> MTEFWLISAPGEKTCQQTWEKLHAATTKNNNLAVSSKFNIPDLKVGTLDVLVGLSDELAKLDAFVEGVVKKVAQYMADVLEDSKDKVQENLLASGVDLVTYITRFQWDMAKYPIKQSLKNISEIIAKGVTQIDNDLKSRASAYNNLKGNLQNLERKNAGSLLTRSLAEIVKKDDFVLDSEYLVTLLVVVPKLNHNDWIKQYETLAEMVVPRSSNVLSEDQDSYLCNVTLFKKAVDDFRHKARENKFIVRDFQYNEEEMRADKEEMNRLSTDKKKQFGPLVRWLKVNFSEAFIAWIHIKALRVFVESVLRYGLPVNFQAMLLQPNKKSVKKLREVLHELYKHLDSSAAAIIDAPMDIPGLNLSQQEYYPYVYYKIDCNLLEFK;>M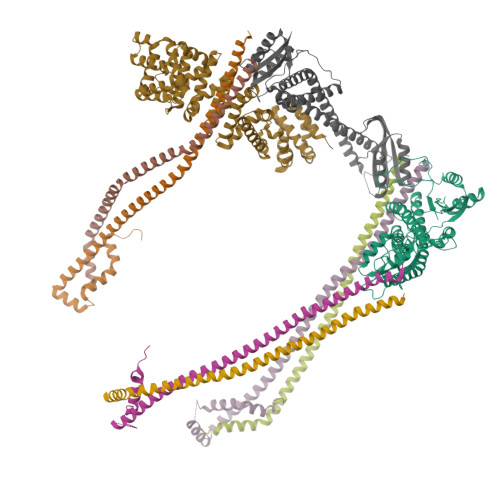ALSDADVQKQIKHMMAFIEQEANEKAEEIDAKAEEEFNIEKGRLVQTQRLKIMEYYEKKEKQIEQQKKIQMSNLMNQARLKVLRARDDLITDLLNEAKQRLSKVVKDTTRYQVLLDGLVLQGLYQLLEPRMIVRCRKQDFPLVKAAVQKAIPMYKIATKKDVDVQIDLEAYLPEDIAGGVEIYNGDRKIKVSNTLESRLDLIAQQMMPEVRGALFGANANRKFLD[3x];>[3x]MASQSQGIQQLLQAEKRAAEKVADARKRKARRLKQAKEEAQMEVEQYRREREQEFQSKQQAAMGSQGNLSAEVEQATRRQVQGMQSSQQRNRERVLTQLLGMVCDVRPQVHPNYRITV;> MTKMDIRGAVDAAVPTNIIAAKAAEVRANKVNWQSYLQGQMISAEDCEFIQRFEMKRCSEEKQEMLQTEGSQCAKTFINLMTHISKEQTVQYILTMVDDMLQENHQRVSIFFDYAKRSKSTAWPYFLPMLNRQDPFTVHMAARIIAKLAAWGKELMEGSDLNYYFNWIKTQLSSQKLRGSGVAVETGTISASDSSQYVQCVAGCLQLMLRVNEYRFAWVEADGVNCIMGVLSNKCGFQLQYQMIFSIWLLAFSPQMCEHLRRYNIIPVLSDILQESVKEKVTRIILAAFRNFLEKSTERETRQEYALAMIQCKVLKQLENLEQQKYDDEDISEDIKFLLEKLGESVQDLSSFDEYSSELKSGRLEWSPVHKSEKFWRENAVRLNEKNYELLKILTKLLEVSDDPQVLAVAAHDVGEYVRHYPRGKRVIEQLGGKQLVMNHMHHEDQQVRYNALLAVQKLMVHNWEYLGKQLQSEQPQTAAARS;> MGELFRSEEMTLAQLFLQSEAAYCCVSELEELGKVQFRDLNPDVNVFQRKFVNEVRRCEEMDRKLRFVEKEIRKANIPIMDTGENPEVPFPRDMIDLEANFEKIENELKEINTNQEALKRNFLELTELKFILRKTQQFFDEMADPDLLEESSSLLEPNEMGRGAPLRLGFVAGVINRERIPTFERMLWRVCRGNVFLRQAEIENPLEDPVTGDYVHKSVFIIFFQGDQLKNRVKKICEGFRASLYPCPETPQERKEMASGVNTRIDDLQMVLNQTEDHRQRVLQAAAKNIRVWFIKVRKMKAIYHTLNLCNIDVTQKCLIAEVWCPVTDLDSIQFALRRGTEHSGSTVPSILNRMQTNQTPPTYNKTNKFTHGFQNIVDAYGIGTYREINPAPYTVITFPFLFAVMFGDFGHGILMTLFAVWMVLRESRILSQKNENEMFSMVFSGRYIILLMGLFSIYTGLIYNDCFSKSLNIFGSSWSVRPMFTIGNWTEETLLGSSVLQLNPAIPGVFGGPYPFGIDPIWNIATNKLTFLNSFKMKMSVILGIIHMLFGVSLSLFNHIYFKKPLNIYFGFIPEIIFMSSLFGYLVILIFYKWTAYDAHSSRNAPSLLIHFINMFLFSYPESGNAMLYSGQKGIQCFLIVVAMLCVPWMLLFKPLILRHQYLRKKHLGTLNFGGIRVGNGPTEEDAEIIQHDQLSTHSEDAEEPTEDEVFDFGDTMVHQAIHTIEYCLGCISNTASYLRLWALSLAHAQLSEVLWTMVIHIGLHVRSLAGGLGLFFIFAAFATLTVAILLIMEGLSAFLHALRLHWVEFQNKFYTGTGFKFLPFSFEHIREGKFDE> GIDPFTGIDPFTKFFYSDQNVDSRDPVQLNLLYVQARDDILNGSHPVSFEKACEFGGFQAQIQFGPHVEHKHKPGFLDLKEFL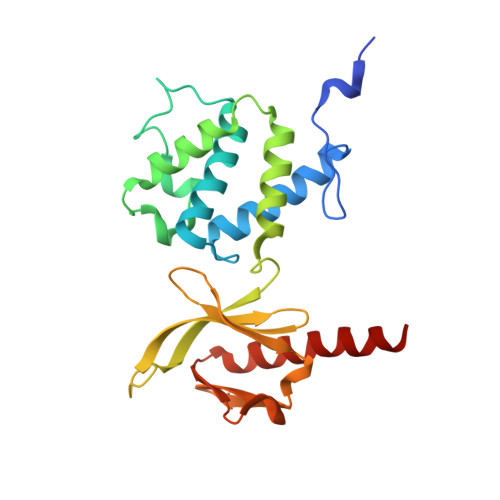PKEYIKQRGAEKRIFQEHKNCGEMSEIEAKVKYVKLARSLRTYGVSFFLVKEKMKGKNKLVPRLLGITKDSVMRVDEKTKEVLQEWPLTTVKRWAASPKSFTLDFGEYQESYYSVQTTEGEQISQLIAGYIDIILKKKQS> PVVIKTEGPAWTPLEPKLITRLADTVRTKGLRSPITMAEVEALMSSPLLPHDVTNLMRVILGPAPYALWMDAWGVQLQTVIAAATRDPRHPANGQGRG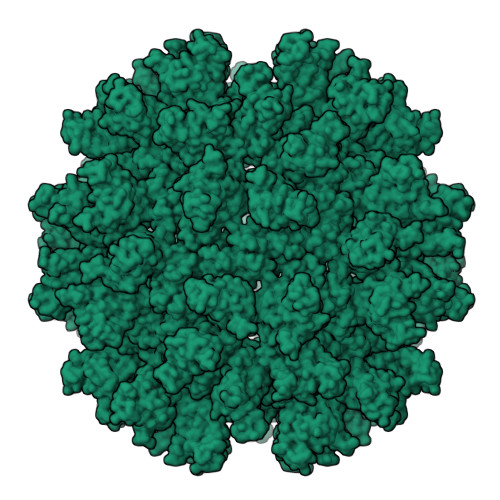ERTNLNRLKGLADGMVGNPQGQAALLRPGELVAITASALQAFREVARLAEPAGPWADIMQGPSESFVDFANRLIKAVEGSDLPPSARAPVIIDCFRQKSQPDIQQLIRTAPSTLTTPGEIIKYVLDRQKTA> DESD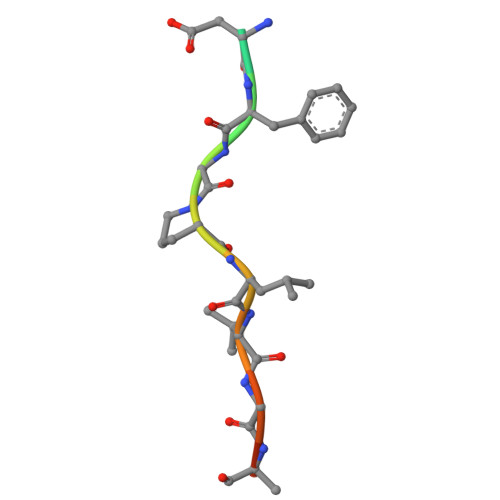FGPLVGADS>[4x]TGNLVTKNSLTPDVRNGIDFKIADLSLADFGRKELRIAEHEMPGLMSLRREYAEVQPLKGARISGSLHMTVQTAVLIETLTALGAEVRWASCNIFSTQDHAAAAVVVGP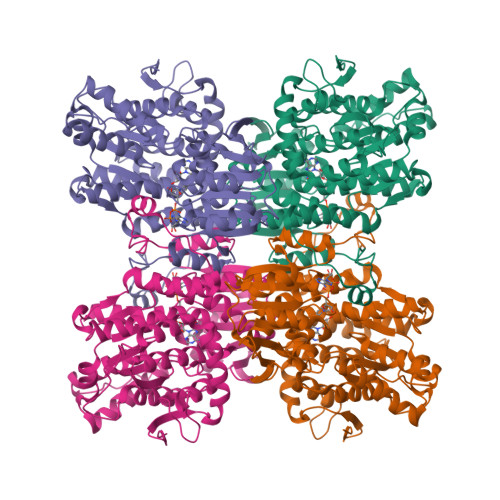HGTPDEPKGVPVFAWKGETLEEYWWAAEQMLTWPDPDKPANMILDDGGDATMLVLRGMQYEKAGVVPPAEEDDPAEWKVFLNLLRTRFETDKDKWTKIAESVKGVTEETTTGVLRLYQFAAAGDLAFPAINVNDSVTKSKFDNKYGTRHSLIDGINRGTDALIGGKKVLICGYGDVGKGCAEAMKGQGARVSVTEIDPINALQAMMEGFDVVTVEEAIGDADIVVTATGNKDIIMLEHIKAMKDHAILGNIGHFDNEIDMAGLERSGATRVNVKPQVDLWTFGDTGRSIIVLSEGRLLNLGNATGHPSFVMSNSFANQTIAQIELWTKNDEYDNEVYRLPKHLDEKVARIHVEALGGHLTKLTKEQAEYLGVDVEGPYKPDHYRY>GPHMENLYFQGGRGVQRKYNIYVALMHYPMRDKEGKVVTTSITNMDLHDISRSCRTFGVKNYFVVNPMPAQREIASRVVRHWIKGYGATYNENRKEAFEYTIITDSLASVIKSIEEKESGSPIIIATTARYQQKAISIEKLKEIADRPILLLFGTGWGFVDDILEF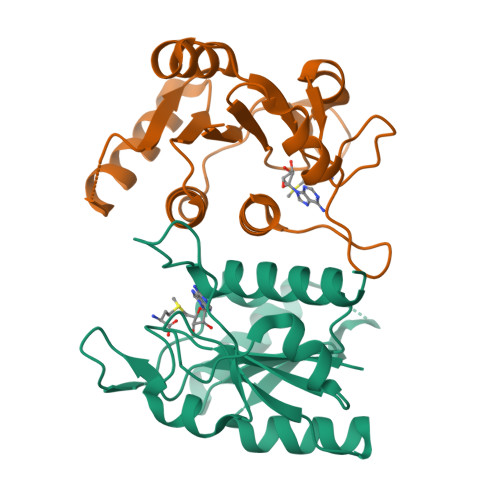ADYVLKPIHGVGDFNHLSVRSAVAIYLDRINRSFQEDIL[2x]>HHHHHHENLYFQSMAVSPSPLRIFTAGGTIDKDFRLEENGLVVGDPFVAEVLKTARLAGAVSIVALSRKDSLDFTEADREAIGRAVGQAVEDHILLTHGTDTMVETARYLGGLPELAGKTVVLSGAMVPGRVGGSDAAFNIGFACAAALMLAPGVYIAMHGKVFDPAKTRKNRGLGRFEPIDDQE[4x]

L‐Asparaginases (ASNases) catalyze the hydrolysis of L‐Asn to L‐Asp and ammonia. In contrast, the chain of ASNase from Rhodospirillum rubrum, reported here and referred to as RrA, consists of only 172 amino acid residues. RrA is homologous to the N‐terminal domain of typical bacterial class 1 ASNases and exhibits millimolar affinity for L‐Asn. Crystal structures of the wild‐type RrA, both with and without bound L‐Asp, as well as structures of several RrA mutants, reveal topologically unique tetramers.

Based on the previously published results for typical class 1 ASNases (Derst et al., 1994; Schalk et al., 2016), we tested two mutants, RrA(Y21A) and RrA(Y21F). When crystallization was done in the presence of L‐Asp, the ligand was present in three out of four protomers and the main chain became fully ordered. As expected, the phenyl group of Phe21 occupied almost exactly the same position as Tyr21 in RrA(wt), leaving no room for any water molecule(s). L‐Asp was bound predominantly by one chain, except that a hydrogen bond was made between its amino nitrogen and the OD2 oxygen of Asn26 of the adjacent protomer. Although both were less active than RrA(wt), RrA(Y21F) is somewhat more active than RrA(Y21A), which is opposite to the results obtained for typical class 1 ASNases. While it is quite plausible that in RrA Tyr21 contributes to proton transfer from the primary nucleophile (Thr16), almost certainly its side chain also contributes to stabilization of the tetramer. In this role, substituting Tyr with Phe preserves this role better than the mutation Tyr → Ala.>[2x]MVPISPIETVPVKLKPGMDGPKVKQWPLTEEKIKALVEICTEMEKEGKISKIGPENPYNTPVFACKKKDSTKWRKLVDFRELNKRTQDFWEVQLGIPHPAGLKKKKSVTVLDVGDAYFSVPLDEDFRKYTAFTIPSINNETPGIRYQYNVLPQGWKGSPAIFQSSMTKILEPFKKQNPDIVIYQYMDDLYVGSDLEIGQHRTKIEELRQHLLRWGLTTPDKKHQKEPPFLWM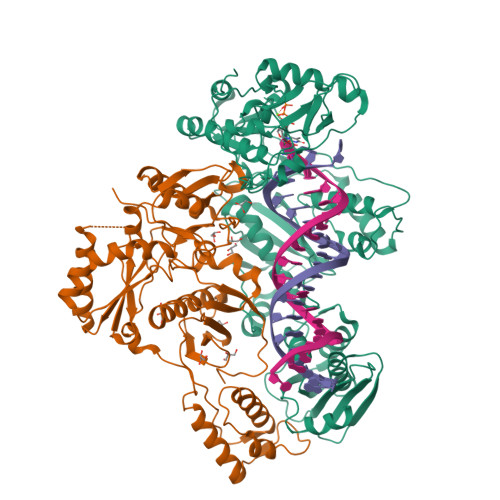GYELHPDKWTVQPIVLPEKDSWTVNDIQKLVGKLNWASQIYPGIKVRQLSKLLRGTKALTEVIPLTEEAELELAENREILKEPVHGVYYDPSKDLIAEIQKQGQGQWTYQIYQEPFKNLKTGKYARMRGAHTNDVKQLTEAVQKITTESIVIWGKTPKFKLPIQKETWETWWTEYWQATWIPEWEFVNTPPLVKLWYQLEKEPIVGAETFYVDGAANRETKLGKAGYVTNKGRQKVVPLTNTTNQKTELQAIYLALQDSGLEVNIVTDSQYALGIIQAQPDKSESELVNQIIEQLIKKEKVYLAWVPAHKGIGGNEQVDKLVSA;>MAHHHHHHALEVLFQGPISPIETVPVKLKPGMDGPKVKQWPLTEEKIKALVEICTEMEKEGKISKIGPENPYNTPVFAIKKKDSTKWRKLVDFRELNKRTQDFWEVQLGIPHPAGLKKKKSVTVLDVGDAYFSVPLDEDFRKYTAFTIPSINNETPGIRYQYNVLPQGWKGSPAIFQSSMTKILEPFKKQNPDIVIYQYMDDLYVGSDLEIGQHRTKIEELRQHLLRWGLTTPDKKHQKEPPFLWMGYELHPDKWTVQPIVLPEKDSWTVNDIQKLVGKLNWASQIYPGIKVRQLSKLLRGTKALTEVIPLTEEAELELAENREILKEPVHGVYYDPSKDLIAEIQKQGQGQWTYQIYQEPFKNLKTGKYARMRGAHTNDVKQLTEAVQKITTESIVIWGKTPKFKLPIQKETWETWWTEYWQATWIPEWEFVNTPPLVKLWYQ[2x]> SMSLAATAWQRLEALFHRACQLPAAEREAFARAQAGDDASLRDDLLAMLAVESQATLRVRAPLKQAVAALRAPLPELPAGTRFGAWAIDRLIGAGGMGQVYLGHRADGAYEREVAIKLVAADALDAQGRALFEFECRLLAQMVHPAIAQIHDVGTDAHGQPYLVAEYLRGEPIT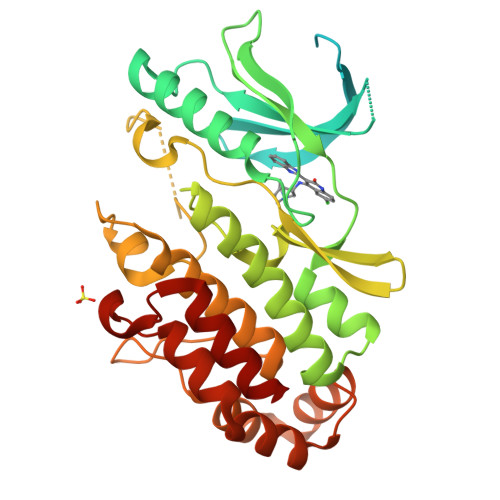WWCDEHRLSLHARVLLMLRVGEAVQHAHQKGVIHRDLKPSNVLVSEIDGRPMPGVIDFGIAVDATNPGMTYAHDRGTPGYMSPEQARGAQDVDARSDIYALGAMFYELSCGLAPVAGRDGVPQPPSQRVAAVPADARARICAARATTYQKLHEQLRDGLDAIVLRALEPQPGARYASVSALLDDLHRWLD> MAPPAKRAKRGWVPPGYKYLGPGNSLDQGEPTNPSDAAAKEHDEAYDQYIKSGKNPYLYFSPADQRFIDQTKDAKDWGGKVGHYFFRTKRAFAPKLSTDSEPGTSGVSRPGKRTKPPAHIFVNQARAKKKRASLAAQQRTLTMSDGTETNQPDTGIANARVERSADGGGSSGGGGSGGGGIGVSTGTYDNQTTYKFLGDGWVEITAHASRLLHLGMPPSENYCRVTVHNNQTTGHGTKVKGNMAYDDTHQQIWTPWSLVDANAWGVWFQPSDWQFIQNSMESLNLDSLSQELFNVVVKTVTEQQGAGQDAIKVYNNDLTACMMVALDSNNILPYTPAAQTSETLGFYPWKPTAPAPYRYYFFMPRQLSVTSSNSAEGTQITDTIGEPQALNSQFFTIENTLPITLLRTGDEFTTGTYIFNTDPLKLTHTWQTNRHLGMPPRITDLPTSDTATASLTANGDRFGSTQTQNVNYVTEALRTRPAQIGFMQPHDNFEANRGGPFKVPVVPLDITAGEDHDANGAIRFNYGKQHGEDWAKQGAAPERYTWDAIDSAAGRDTARCFVQSAPISIPPNQNQILQREDAIAGRTNMHYTNVFNSYGPLSAFPHPDPIYPNGQIWDKELDLEHKPRLHVTAPFV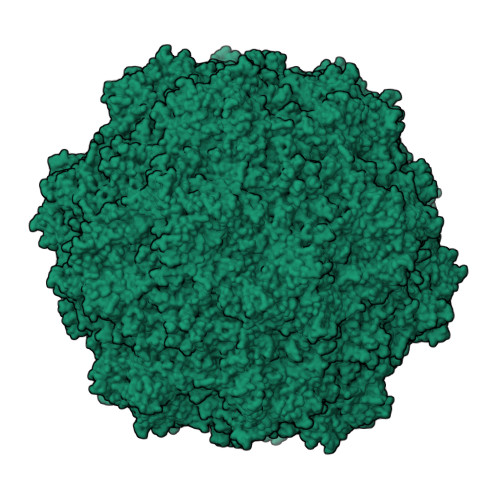CKNNPPGQLFVRLGPNLTDQFDPNSTTVSRIVTYSTFYWKGILKFKAKLRPNLTWNPVYQATTDSVANSYMNVKKWLPSATGNMHSDPLICRPVPHMTY> MKTITGVFNSFDSLTWTRSVEYVYKGPETPTWNAVLGWSLNSTTADPGDTFTLILPCVFKFITTQTSVDLTADGVSYATCDFNAGEEFTTFSSLS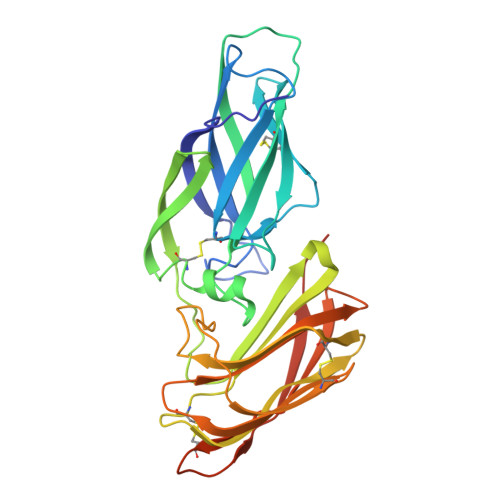CTVNSVSVSYARVSGTVKLPITFNVGGTGSSVDLADSKCFTAGKNTVTFMDGDTKISTTVDFDASPVSPSGYITSSRIIPSLNKLSSLFVVPQCENGYTSGIMGFVASNGATIDCSNVNIGISKGLNDWNFPVSSESFSYTKTCTSTSITVEFQNVPAGYRPFVDAYISAENIDKYTLTYANEYTCENGNTVVDPFTLTWWGYKNSEADSDGDVIVV> Q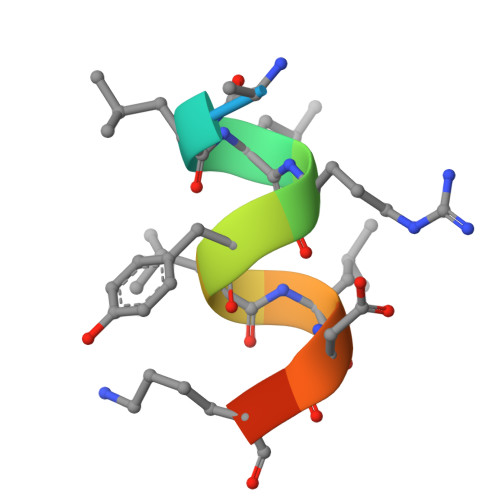ALLRYLLDKDD> GSHMGSNQKRGVKVLKQELGGLGISIKGGKENKMPILISKIFKGLAADQTQALYVGDAILSVNGADLRDATHDEAVQALKRAGKEVLLEVKYMREGSAYGSVKAYTNFDAERDALNIETAIKTKGVDEVTIVNILTNRSNEQRQDIAFAYQRRTKKELASALKSALSGHLETVILGLLKTPAQYDASELKASMKGLGTDEDSLIEIICSRTNQELQEINRVYKEMYKTDLEKDIISDTSGDFRKLMVALAKGRRAEDG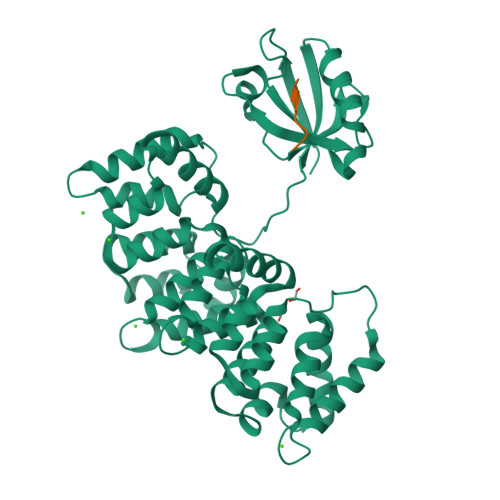SVIDYELIDQDARDLYDAGVKRKGTDVPKWISIMTERSVPHLQKVFDRYKSYSPYDMLESIRKEVKGDLENAFLNLVQCIQNKPLYFADRLYDSMKGKGTRDKVLIRIMVSRSEVDMLKIRSEFKRKYGKSLYYYIQQDTKGDYQKALLYLCGGDD;> SEKHFRETEV>MGPLTESYCGPCPKNWICYKNNCYQFFDEEKNWYESQAS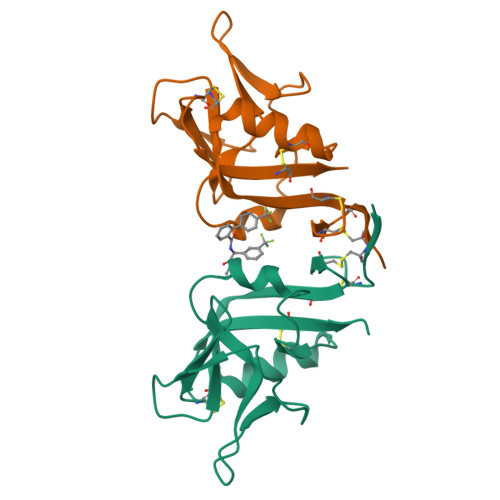CMSQNASLLKVYSKEDQDLLKLVKSYHWMGLVHIPTNGSWQWEDGSSLSPNLLTIIEMQKGDCALYASSFKGYIENCSTPNTYICMQRTV[2x]Here, we report the atomic structures of an engineered diffocin, a contractile syringe-like molecular machine that kills the Gram-positive bacterium Clostridioides difficile. Captured in one pre-contraction and two post-contraction states, each structure fashions six proteins in the bacteria-targeting baseplate, two proteins in the energy-storing trunk, and a collar linking the sheath with the membrane-penetrating tube. Specific attachment of baseplate tail fibers to receptors on the surface of a target bacterial cell triggers conformational changes of the neighboring baseplate, which leads to reorientation of sheath proteins and contraction of the entire sheath assembly. Since the sheath and the tube are anchored together at the opposite end by the collar, collapsing the sheath pushes the tube through the baseplate, driving it to puncture the cell wall and underlying cytoplasmic membrane.

The diffocin baseplate has an inner section that connects to the tube and an outer section that connects to the sheath. The outer section of the baseplate consists of sheath initiator (CD1370) and triplex proteins (CD1371 and CD1372). Two conformers of CD1371, Tri2A and Tri2B, and one of CD1372, Tri1, form the triplex, and six copies of the triplex form the baseplate wedge, surrounding the inner baseplate. Within each triplex, the N-terminal regions of the three subunits form a core bundle and a trifurcation unit, from which the C-terminal dimerization domains of Tri2A and Tri2B extend in opposite directions to interact with neighboring triplexes. The C-terminal region of Tri1, along with the tail fiber linked to it, was not resolved in the cryoEM maps. Notably, both Tri2A and Tri2B include a wing domain inserted between the core bundle and the trifurcation unit, reminiscent of gp6 in phage T412. These wing domains contribute to the interface with the hydrolase domain of the hub-hydrolase. The hydrolase domain has a dumbbell shape, with its two lobes binding to the peripheral region of the baseplate wedge. Given that the local resolution of the peripheral region of the baseplate is only sufficient to assign secondary structural elements, the model of the hydrolase domain and surrounding triplex motifs were built with the assistance of AlphaFold225. The N-terminal domain (residues 49–105) of the sheath initiator binds to the core bundle of the triplex, while the C-terminal β-hairpin (residues 106–135) interacts with two sheath proteins on the first sheath layer by forming a conserved handshake interface.

>MYSDQTYEVIKNRTLENINLDIYKGEGSFLNNMVSGNNLELSKIYLELSKMHKMAFIQDTYNQFLDKRVNEFGVYRKLGTESNGEVEFIGEKGTVINNGTIISYRDLLFVVIKDVTIGSEEGDNSPVQALEVGKKYNLPTNCEFKLVDNISGVTKITNTRSFEGGTDIETDEELKERFYKIQRNQATSGNKAHYEEWALEVDGVYNVKVYPRWDGPGTVKVLIFGKNNQAVDTETIERCQQHIDEEKPIGPTITVVTPLPIEISISAVMKLEDGYTLDNVKESFLESINTYFRDIRGEIIYTKVMGILINTTGVHDLSNLLINGSTDNITINEDKIPSVTTVNFSEVENQ[12x];>MAIGLPSINISFKELATTVKERSARGIIAMVLKDAKALGLNEIHEKEDIPVDLSAENKEYINLALMGNVNTPNKLLVYVIEGEADIQTALDFLETKEFNYLCMPKAVEADKTAIKNWIIKLRDIDKVKVKAVLGKVVGNHEGIINFTTEDVLVGEKKYSVDEFTSRVAGLIAGTPLSQSVTYTKLSDVVDIPKMTKVDAESRVNKGELILIKEAGAIRIARGVNSLTELTAEKGEMFQKIKIVDTLDIIHSDIRKVIIDDYIGKVTNSYDNKCLLIVAIKSYLEELEKSALIESDSTVEIDFEAQKSYLKSKGVDLSYMTLQEIKEANTGSKVFLKAKIKVLDAMEDIDLSIEI[12x];>[6x]MSTIFPFIGVPEDYILPKTEELPIFREVAWDFEKDEPILEKGDFKIIEKKEALKVWIYKCIKTNRYEHEIYSLEYGTELSELIGQKYTKGLTESEASRFIKEALLINPYILEVNVKSANFNRDILSANVKVSTIYGEVEINV;>MKLIDKLPSFDRNYIVEEIQGAYDTELNILKEDIDDTFNQLFVDTATWGLDMWEDILCIEKKELDFDTRRSNIKAKMRSRGTSTIEVIKSICEAYTKSETDIKVYSDEFTFVLSFIANNCDYKTLLDCSDMIERVKPAHLLHYLEPIILDKSMVYCGGGMVCSEEVKVHPYFEPIIKCSAVVNCGAGMISREEIKVYPLSIKCIENNCKINIAIANDTGVENVVVYPKSEVV[6x];>[12x]MANMEARNVMSGTWGELWLDGNKVAEVKKFQAKMEFTKEDIIIAGQMGTDTKYMGYKGKGSITLYHVSSRMHKLIGEKIKRGSEPRFVAISKLNDPDSYGAERIAVKNIAFDDLTLADWEVGVKGEIEAPFTFTEYDFLDII;>MGNVREEGINMYLTDNYTPKMNQIISVTDNFRRATVAVSLSTNVMASSIKNSIGSASNRVNSLNSSLRKVQTTASSVSSTMTKLSSSINAVSGVIGSLNGSIMRLAITIAMIIDYFNKLIQKKNEFNSNIMIILIFKAKSDEVEKTKNKLLGNLKKIGGKIWNIVIKAKDMTKRVISSILGKLKQVEKRPYQGSINLKDMVSSAMGRILPKLMLFKNTFWSGVIAIKDMASGIISKVFPKLRLFAGKVWSGAIAVKDMASGILGSIKGKISDLTNGATIGVAVKKGVDLLGQEQNQKVVLESVMKRNTGKVNQIDVDDYYGSLVRMANDTPFDPEDVVAMGTKAKMISNITGGKKEKDITQAMVDVRALNMNTSSEQDVSAAFLSAAKGNMESLNTLVGENYKTFDEALEGISVKQMGLAKEMSNTIPGIISGAQTSINNGLKSIVKPFDDILGQGLKKIKTFIESGLGNLAGLSEKMAGKIGNVMNGKIIIGNKYDQMQSRSVKNGKEFSDSTQYRISNEAEKRKMMVENKQERFENHAATMIGNAPKAIVNAGSTLLQNIDFTALIDSLLPVVNLVNNLLDSINNKSPIAQGLISIFGTIVTTAFQLIGPVVEAVSPIITRIFTFLGEYAPQINNFIETLGVIWKTVWETLGPLLETGWKIIEPILGAFFNILDKVCKIVKDICKWWQTMINKIKNGSITGTVLNLVEKSKKNYKDNPYAGTKAGDSGKAYSGKKGNNAFGLNYVPYNDYQTRLHEGEMVLTKQEANQYRSRKNGGNINIAKLADTIVIREEADIEKITSKLVASIQLAQLGGVL[3x];>MANPINEFIGIIREEGKYHNQPSFFIGKIKSKLPDLKIETNNIILEKEDILIDSWMIDRQLETFDTETNQEHQHEVKNPFIDNFESGDMVIMFRIGEKFAVVSKLVSL[3x];>[6x]MEMWLRQAEDRFRFPVFPSSFSINGKAAVNSSSILKIGEIATFGGVALKSISISSFFPNKDYTFCDYTGFPSPYDCVNKIEKWMKEGFILRFTITETNINMEVIIEGFSYEERDGTRDVYFTLDLKEYKRIKIPKVTPKQ;>MIKIWVHIKNGSIYDITDIVDKVSWSGDYKSPSRTLEFSIIQSSFDNVFQQIDIPIASTVCFYVDEKELFRGMIINRSKDSSSNEISFVSKDMGFLLTQSEVSYNFKDKLVEDIAKQVFAENRLSVGIIAKTNVKYTKMFIGVNGYDTIMSAYTEASKKTKKKYMIEANLDKFNVIEKGTVTLSVMFEEGFNIINTTFSESMENVKNKVIVVDQYGSKISEKIDNEIFKEVNVIMQKVIQQQENQDVDIDSEFNGIEKSCSLKGYGDVSCITGRGVKVKDSYTKLVGLFYIDTDKHTWQNGEYQIELELNFQNLMDEKSAGQDEPKEESNLGGEDYAGGKEFTAEFTAYCPRKEEGGDTDCRKKKLDPSKKTCAAPMVGKYEQTYYTKEFLNKHPLLNYGDEIQVITGVSGRDGVYKVNDVGPAITIEKNGTYHIDILFGNVEEASKFGRRKGKIIIGGYSGNVSDKAKIVISEAKKHLGKPYKWGGNGPSSFDCSGLMVYCFKKVNVSLPRTSNQQSKKGKKVEQKNLQAGDLVFFHNPVSHVGLYIGNGEFLHAPQKGDVVKISKLSSRRDFNTARRVL[3x]> MIVLFVDFDYFYAQVEEVLNPSLKGKPVVVCVFSGRFEDSGAVATANYEARKFGVKAGIPIVEAKKILPNAVYLPMRKEVYQQVSSRI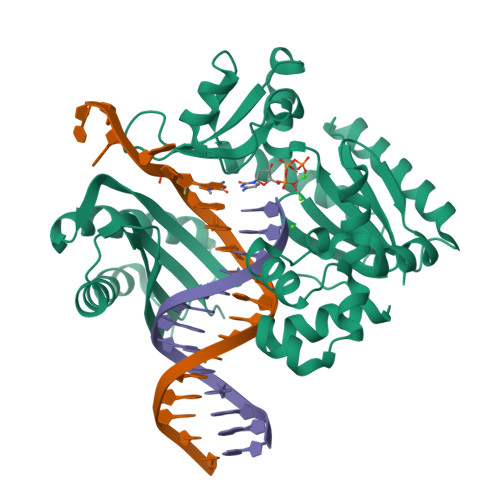MNLLREYSEKIEIASIDEAYLDISDKVRDYREAYNLGLEIKNKILEKEKITVTVGISKNKVFAKIAADMAKPNGIKVIDDEEVKRLIRELDIADVPGIGNITAEKLKKLGINKLVDTLSIEFDKLKGMIGEAKAKYLISLARDEYNEPIRTRVRKSIGRIVTMKRNSRNLEEIKPYLFRAIEESYYKLDKRIPKAIHVVAVTEDLDIVSRGRTFPHGISKETAYSESVKLLQKILEEDERKIRRIGVRFSKFI> AHKAQQYYFDAAEAEAWMSEQELYMMSEEKAKDEQSAVS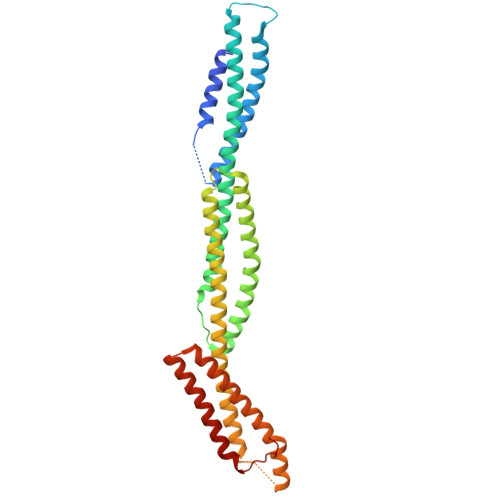MLKKHQILEQAVEDYAETVHQLSKTSRALVADSHPESERISMRQSKVDKLYAGLKDLAEERRGKLDERHRLFQLNREVDDLEQWIAEREVVAGSHELGQDYEHVTMLQERFREFARDTGNIGQERVDTVNNMADELINSGHSDAATIAEWKDGLNEAWADLLELIDTRTQILAASYELHKFYHDAKEIFGRIQDKHKKLPEELGRDQNTVETLQRMHTTFEHDIQALGTQVRQLQEDAARLQAAYAGDKADDIQKRENEVLEAWKSLLDACEGRRVRLVDT>EVKLILYHWTHSFSSQKVRLVIAEKALKCEEHDVSLPLSEHNEPWFMRLNSTGEVPVLIHGENIICEATQIIDYLEQTFLDERTPRLMPDKESMYYPRVQHYRELLDSLPMDAYTHGCILHPELTVDSMIPAYATTRIRSQIGNTESELKKLAEENPDLQEAYIAKQKRLKSKLLDHDNVKYLKKILDELEKVLDQVETELQRRNEETPEEGQQPWLCGESFTLADVSLAVTLHRLKF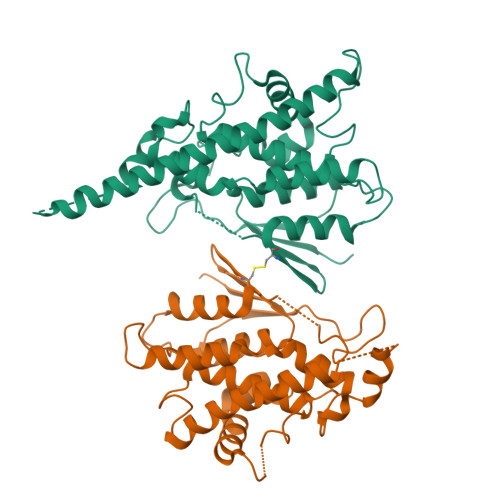LGFARRNWGNGKRPNLETYYERVLKRKTFNKVLGHVNNILIS[2x]>[3x]MSNPTKISILGRESIIADFGLWRNYVAKDLISDCSSTTYVLVTDTNIGSIYTPSFEEAFRKRAAEITPSPRLLIYNRPPGEVSKSRQTKADIEDWMLSQNPPCGRDTVVIALGGGVIGDLTGFVASTYMRG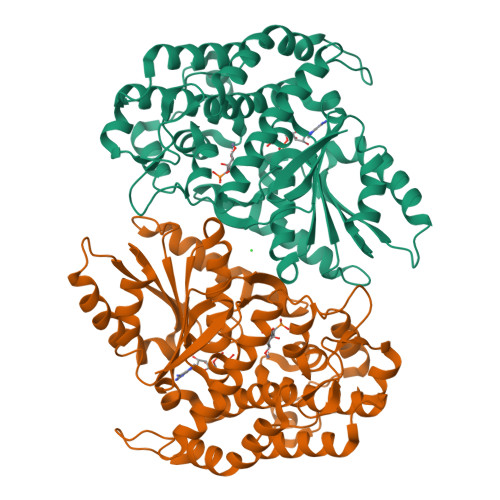VRYVQVPTTLLAMVDSSIGGKTAIDTPLGKNLIGAIWQPTKIYIDLEFLETLPVREFINGMAEVIKTAAISSEEEFTALEENAETILKAVRREVTPGEHRFEGTEEILKARILASARHKAYVVSADEREGGLRNLLNWGHSIGHAIEAILTPQILHGECVAIGMVKEAELARHLGILKGVAVSRIVKCLAAYGLPTSLKDARIRKLTAGKHCSVDQLMFNMALDKKNDGPKKKIVLLSAIGTPYETRASVVANEDIRVVLAP> KGPNGLIERQVTRELLELFNIDEQTLNTQGLVVTTTIDPQAQRAAEKAVAKYLDGQDPDMRAAVVSIDPHNGAVRAYYGGDNANGFDFAQAGLQTGSSFK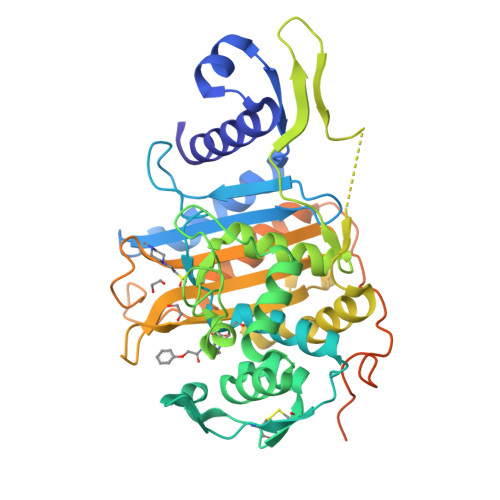VFALVAALEQGIGLGYQVDSSPLTVDGIKITNVEGEGCGTCNIAEALKMSLNTSYYRLMLKLNGGPQAVADAAHQAGIASSFPGVAHTLSEDGKGGPPNNGIVLGQYQTRVIDMASAYATLAASGIYHPPHFVQKVVSANGQVLFDASTADNTGDQRIPKAVADNVTAAMEPIAGYSRGHNLAGGRDSAAKTGTTQFGDTTANKDAWMVGYTPSLSTAVWVGTVKGDEPLVTASGAAIYGSGLPSDIWKATMDGALKGTSNETFPKPTEVGGYAGVPPPPPPPEVPPSETVIQPTVEIAPGITIPIGPPTTITLAPPPPAPPAATPTPPP(2R)-N-(2H-indazol-4-yl)-1-[1-(4-methoxyphenyl)cyclopentyl]carbonyl-pyrrolidine-2-carboxamide 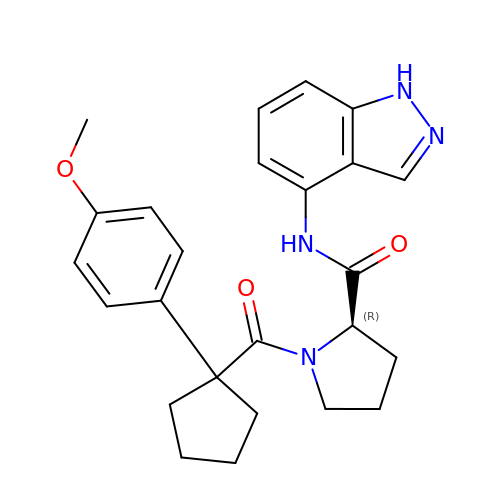| C25 H28 N4 O3 | KRGAGJKQQRBFEC-JOCHJYFZSA-N>MVPAAQQTATAPDAALTFPEGFLWGSATASYQIEGAAAEDGRTPSIWDTYARTPGRVRNGDTGDVATDHYHRWREDVALMAELGLGAYRFSLAWPRIQPTGRGPALQKGLDFYRRLADELLAKGIQPVATLYHWDLPQELENAGGWPERATAERFAEYAAIAADALGDRVKTWTTLNEPWCSAFLGYGSGVHAPGRTDPVAALRAAHHLNLGHGLAVQALRDRLPADAQCSVTLNIHHVRPLTDSDADADAVRRIDALANRVFTGPMLQGAYPEDLVKDTAGLTDWSFVRDGDLRLAHQKLDFLGVNYYSPTLVSEADGSGTHNSDGHGRSAHSPWPGADRVAFHQPPGETTAMGWAVDPSGLYELLRRLSSDFPALPLVITENGAAFHDYADPEGNVNDPERIAYVRDHLAAVHRAIKDGSDVRGYFLWSLLDNFEWAHGY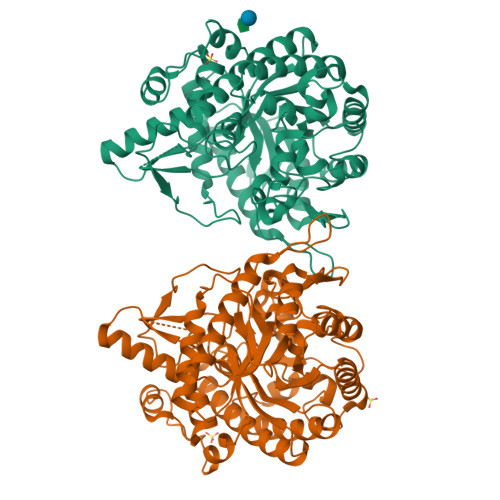SKRFGAVYVDYPTGTRIPKASARWYAEVARTGVLPTA[2x]>[4x]MTSFQEVPL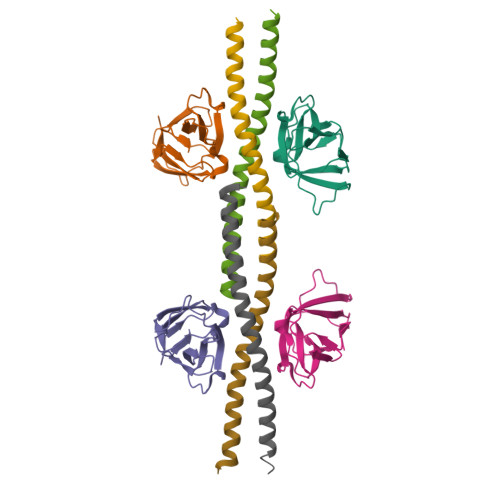QTSNFAHVIFQNVAKSYLPNAHLECHYTLTPYIHPHPKDWVGIFKVGWSTARDYYTFLWSPMPEHYVEGSTVNCVLAFQGYYLPNDDGEFYQFCYVTHKGEIRGASTPFQFR;>[4x]GSEFKENIINDLSDKLKSTMQQQERDKDLIESLSEDRARLLEEKKKLEEEVSKLRSS The mGeos series of rsFP’s display similar switching behavior to Dronpa. The series was developed from mEos2, with mutations that remove the undesirable irreversible green-to-red photo conversation, increase fluorescence brightness and provide high thermal stability of the off-state. Skylan-NS represents a further improvement, with reduced per cycle bleaching and higher photoswitching quantum yield in the on→off than Dronpa. We present high resolution room temperature SFX structures of Skylan-NS in both ‘on’ and meta-stable ‘off’ state collected using two different XFELs, the SPring-8 Angstrom Compact free electron Laser (SACLA), Japan and the Linear Coherent Light Source (LCLS), USA.

We collected datasets for the dark on-state using two different methods at the SACLA/EH4 station using the DAPHNIS chamber. Firstly, by using the grease injection method, we selected relatively large crystals of 50–100 μm in size. Diffraction was collected up to 1.9 Å resolution with diffraction still present in the corners of the detector. The hit-rate could be carefully controlled with the crystal density, and levels of 40% could be sustained with crystal densities of 4.8 × 107–9 × 107 crystal/mL. Table 1 shows the CC* and R-split values that reveal data from the droplet method was lower quality than that obtained from the grease injection method. The comparison between the two on-state structures collected with the grease injection and droplet methods under the same conditions (Black) showed the lowest R-factor over the intermediate resolution range up to ≈3 Å resolution. An increase of the R-factor for the increased resolution (<3 Å) is likely indicative of genuine structural differences between the grease and droplet methods, in agreement with the observed degradation of R-split and CC* when merging intensities together (Black). The dehydrating effect on the crystals due to the mother liquor being replaced with a mineral oil–based grease matrix in the grease injection method could explain this difference. Following complete refinement of all four datasets, both on-state structures showed no statistically significant density in either the 2Fobs-Fcalc or the Fobs-Fcalc maps that could be assigned to a trans chromophore structure. The same was observed for chromophore omit maps, that also, at lower sigma levels, did not show such density. This is in agreement with the dark incubation and dark sample injection which corresponds to a 100% on-state concentration. Photoisomerisation is clearly seen in a comparison of the “on” and “off” refined structures where the dihedral angle of the chain connecting the phenol ring to the rest of the chromophore (N–C=C–C) changes from 1° (cis) → 171.1° (trans) in the on- vs the off-state and the pheonolic oxygen is displaced by 6.2 Å.

> MSAIKPDMKIKLRMEGNVNGHHFVIDGDGTGKPFEGKQSMDLEVKEGGPLPFAFDILTTAFLYGNRVFAKYPDNIQDYFKQSFPKGYSWERSLTFEDGGICNARNDITMEGDTFYNKVRFYGTNFPANGPVMQKKTLKWEPSTEKMYVRDGVLTGDVEMALLLEGNAHYRCDFRTTYKAKEKGVKLPGAHFVDHCIEILSHDKDYNKVKLYEHAVAHSGLPDNARR>[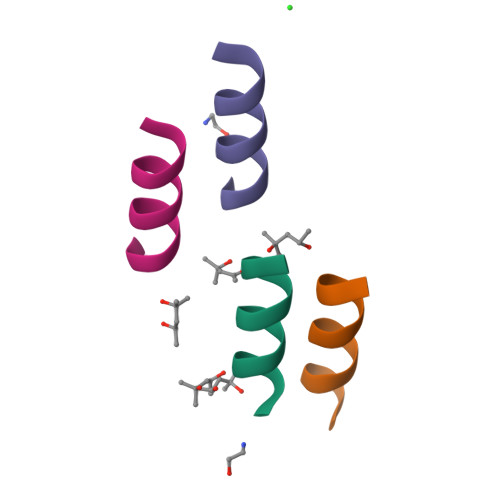4x]XELLKKLLEELKG>[2x]HHHHHHMANLPILLDYWPSMFGMRARVALREKGVEFEYREEDFSNKSPLLLQSNPIHKKIPVLVHNGKPVCESLNVVQYVDEAWPEKNPFFPS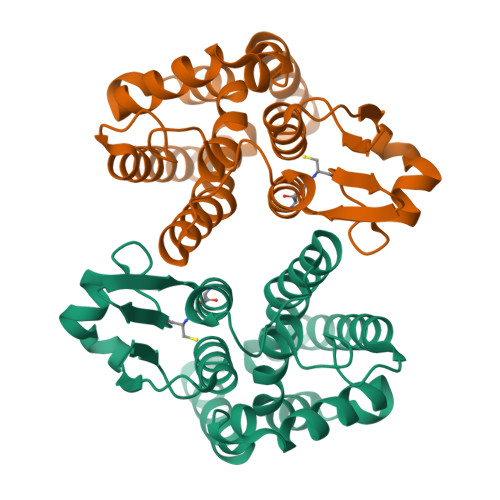DPYGRAQARFWADFVDKKFTDAQFKVWGKKGEEQEAGKKEFIEAVKILESELGDKPYFGGDSFGYVDISLITFSSWFQAYEKFGNFSIESESPKLIAWAKRCMEKESVSKSLPDSEKIVAYAAEYRKNNL> MTGMSREEVESLIQEVLEVYPEKARKDRNKHLAVNDPAVTQSKKCIISNKKSQPGLMTIRGCAYAGSKGVVWGPIKDMIHISHGPVGCGQYSRAGQRNYYIGTTGVNAFVTMNFTSDFQEKDIVFGGDKKLAKLIDEVETLFPLNKGISVQSECPIGLIGDDIESVSKVKGAELSKTIVPVRCEGFRGVSQSLGHHIANDAVRDWVLGKRDEDTTFASTPYDVAIIGDYNIGGDAW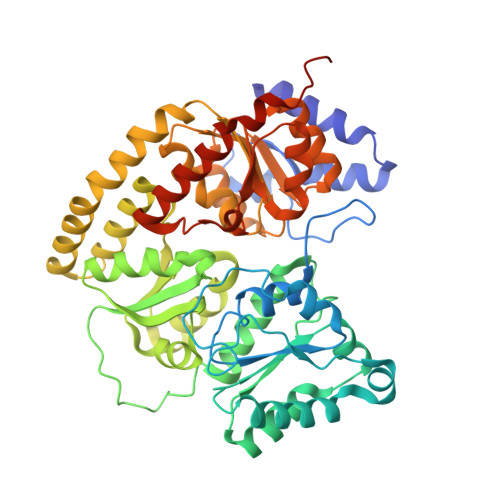SSRILLEEMGLRCVAQWSGDGSISEIELTPKVKLNLVHCYRSMNYISRHMEEKYGIPWMEYNFFGPTKTIESLRAIAAKFDESIQKKCEEVIAKYKPEWEAVVAKYRPRLEGKRVMLYIGGLRPRHVIGAYEDLGMEVVGTGYEFAHNDDYDRTMKEMGDSTLLYDDVTGYEFEEFVKRIKPDLIGSGIKEKFIFQKMGIPFREMHSWDYSGPYHGFDGFAIFARDMDMTLNNPCWKKLQAPWEASEGAEKVAASA> GPLGSKSSQYRKMKTEWKSNVYLARSRIQGLGLYAARDIEKHTMVIEYIGTIIRNEV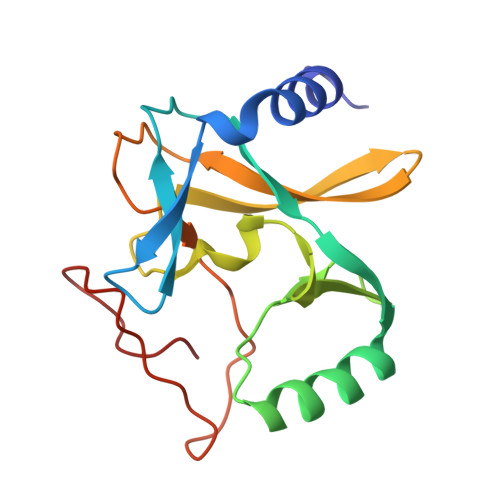ANRKEKLYESQNRGVYMFRMDNDHVIDATLTGGPARYINHSCAPNCVAEVVTFERGHKIIISSSRRIQKGEELCYDYKFDFEDDQHKIPCHCGAVNCRKWMN> MAEVVNGKLHLRFAIAPMRPTPSQTIKEFEPIFKYLADQLGATYEIVSPESWAAISVAMTNGHVDVGWLGPWGYVLSNKKAGTEVLATVKYRGEPFYKALIVGRADLPIKKWPEDAKGLKLSLSDQGNTSGWLIPMAYFKSIGIDPASYFEYREGATFGQNESQIQHGLIDLGS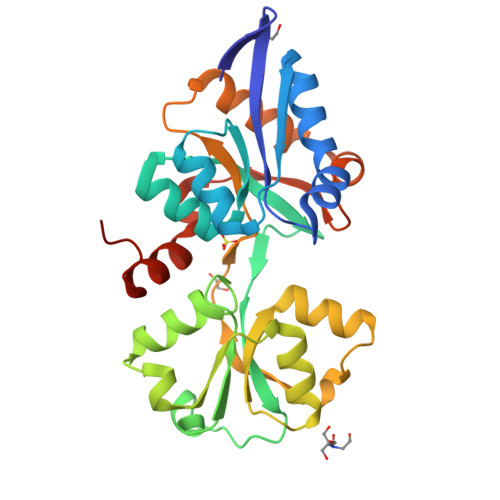DMDRGRNGMIEAGQIDPSKSKIVWESSKLPNNAISVPKDFDPALKARITEILTSLSEEKAQSLMGSGYNGFVKAKHSDYKVIEDAGRILGKLLEHHHHHH> CGUGCUCCCCACCUCGGAUCACUGCG;> GCAGGAACCGAGAGGCAC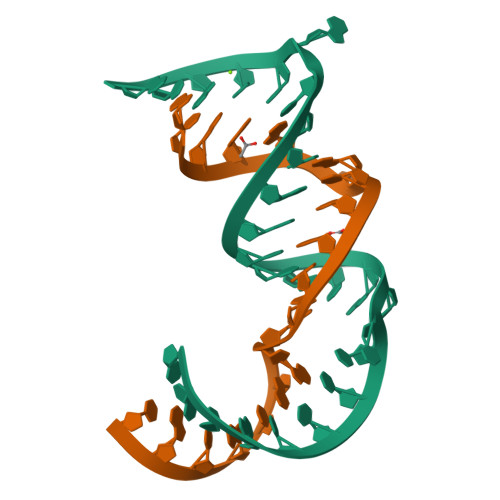GC>[2x]MPLMQGMEVQPHIRLRKEDVEPVVIIVGDPARTEEVANMCEKKQELAYNREYRSFRVVYDSQPITVISHGIGCPGTSIAIEELAYLGAKVIIRAGTCGSLKPKTLKQGDVCVTYAAVNETGLISNILPEGFPCVATPHVYQALMDAAKELGIEAASGIGVTQDYFYQNGILPSKLEMYSKCCDVIDMEMSGVLGLCQARGIATCGILAVDGSPLQ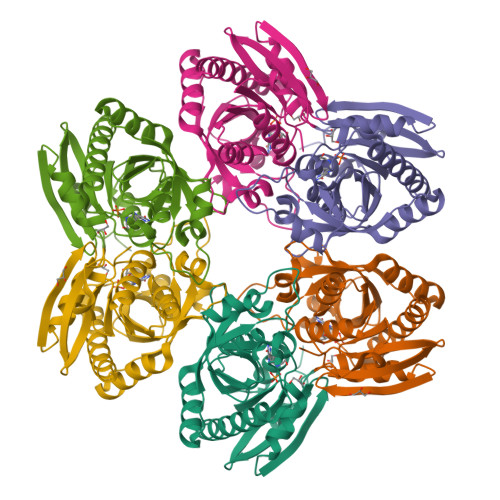WDEGDYDATGVKATTGKENMVKITLKACANLRRQYKGEFEAYVEQKLISEEDLNSAVDHHHHHH>MVSVIKPEMKMRYYMDGSVNGHEFTIEGEGTGRPYEGHQEMTLRVTMAKGGPMPFAFDLVSHVFCYGHRPFTKYPEEIPDYFKQAFPEGLSWERSLEFEDGGSASVSAHISLRGNTFYHKSKFTGVNFPADGPIMQNQSVDWEPSTEKITASDGVLKGDVTMYLKLEGGGNHKCQF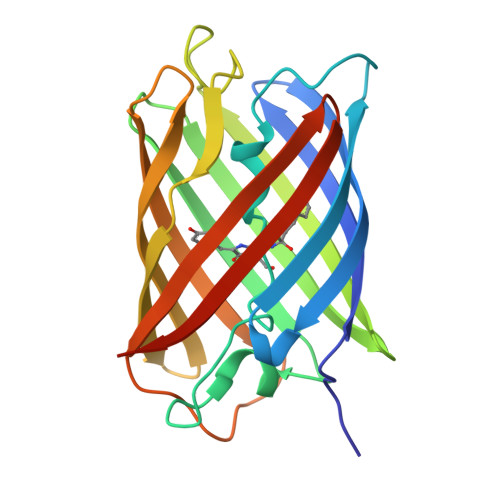KTTYKAAKKILKMPGSHYISHRLVRKTEGNITELVEDAVAHSLEHHHHHH[4x]4-METHYLUMBELLIFERYL-ALPHA-D-GLUCOSE 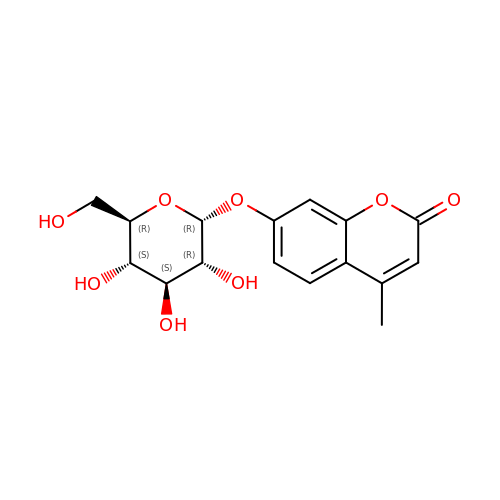| C16 H18 O8 | YUDPTGPSBJVHCN-JZYAIQKZSA-N>[12x]HHHHHHDYKDDDDKLEVLFQGPEFMTSVRCKLAQYLEDLEDVDLKKFKMHLEDYPPEKGCIPVPRGQMEKADHLDLATLMIDFNGEEKAWAMAVWIFAAINRRDLWEKAKKDQPEWNDTCTSHSSMVCQEDSLEEEWMGLLGYLSRISICKKKKDYCKMYRRHVRSRFYSIKDRNARLGESVDLNSRYTQLQLVKEHPSKQEREHELLTIGRTKMRDSPMSSLKLELLFEPEDGHSEPVHTVVFQGAAGIGKTILARKIMLDWALGKLFKDKFDYLFFIHCREVSLRTPRSLADLIVSCWPDPNPPVCKILRKPSRILFLMDGFDELQGAFDEHIGEVCTDWQKAVRGDILLSSLIRKKLLPKASLLITTRPVALEKLQHLLDHPRHVEILGFSEAKRKEYFFKYFSNELQAREAFRLIQENEVLFTMCFIPLVCWIVCTGLKQQMETGKSLAQTSKTTTAVYVFFLSSLLQSRGGIEEHLFSDYLQGLCSLAADGIWNQKILFEECDLRKHGLQKTDVSAFLRMNVFQKEVDCERFYSFSHMTFQEFFAAMYYLLEEEAEGETVRKGPGGCSDLLNRDVKVLLENYGKFEKGYLIFVVRFLFGLVNQERTSYLEKKLSCKISQQVRLELLKWIEVKAKAKKLQWQPSQLELFYCLYEMQEEDFVQSAMDHFPKIEINLSTRMDHVVSSFCIKNCHRVKTLSLGFFHNSPKEEEEERRGGRPLDQVQCVFPDTHVACSSRLVNCCLTSSFCRGLFSSLSTNRSLTELDLSDNTLGDPGMRVLCEALQHP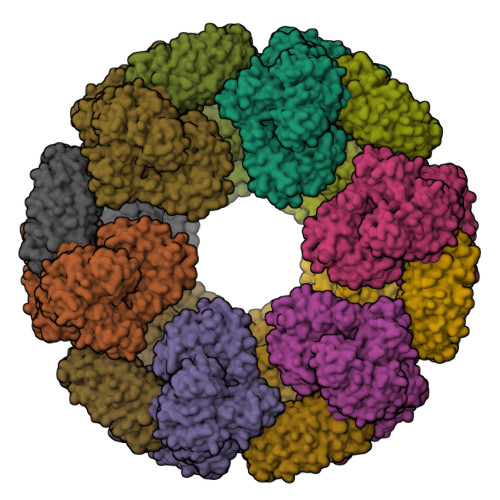GCNIQRLWLGRCGLSHQCCFDISSVLSSSQKLVELDLSDNALGDFGIRLLCVGLKHLLCNLQKLWLVSCCLTSACCQDLALVLSSNHSLTRLYIGENALGDSGVQVLCEKMKDPQCNLQKLGLVNSGLTSICCSALTSVLKTNQNFTHLYLRSNALGDTGLRLLCEGLLHPDCKLQMLELDNCSLTSHSCWNLSTILTHNHSLRKLNLGNNDLGDLCVVTLCEVLKQQGCLLQSLQLGEMYLNRETKRALEALQEEKPELTIVFEISW> MVLMIVSGRSGSGKSVALRALEDMGFYCVDNLPVVLLPDLARTLADREISAAVSIDVRNMPESPEIFEQAMSNLPDAFSPQLLFLDADRNTLIRRYSDTRRLHPLSSKNLSLESAI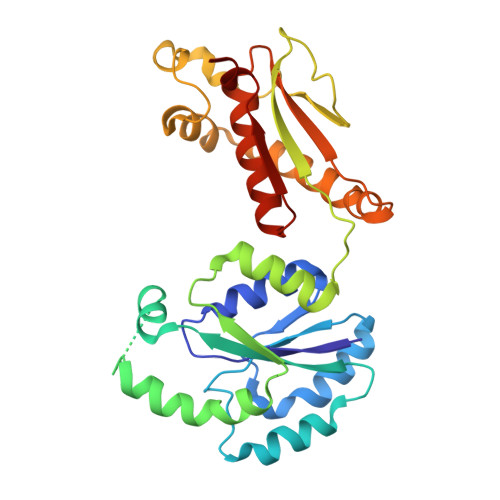DKESDLLEPLRSRADLIVDTSEMSVHELAEMLRTRLLGKRERELTMVFESFGFKHGIPIDADYVFDVRFLPNPHWDPKLRPMTGLDKPVAAFLDRHTEVHNFIYQTRSYLELWLPMLETNNRSYLTVAIGCTGGKHRSVYIAEQLADYFRSRGKNVQSRHRTLEKRKP>[5x]GPAMGYARRVMDGIGEVAVTGAGGSVTGARLRHQVRLLAHALTEAGIPPGRGVACLHANTWRAIALRLAVQAIGCHYVGLRPTAAVTEQARAIAAADSAALVFEPSVEARAADLLERVSVPVVLSLGPTSRGRDILAASVPEGTPLRYREHPEGIAVVAFTSGTTGTPK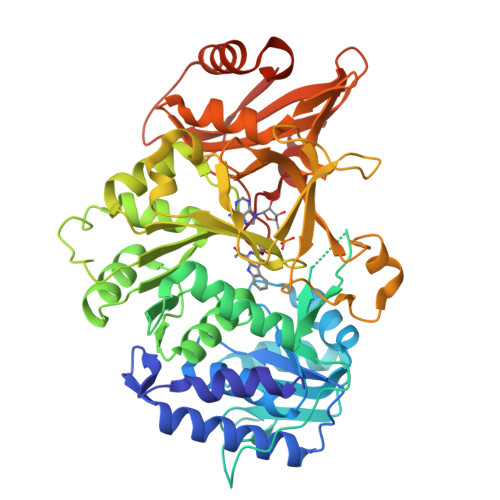GVAHSSTAMSACVDAAVSMYGRGPWRFLIPIPLSDLGGELAQCTLATGGTVVLLEEFQPDAVLEAIERERATHVFLAPNWLYQLAEHPALPRSDLSSLRRVVYGGAPAVPSRVAAARERMGAVLMQNYGTQEAAFIAALTPDDHARRELLTAVGRPLPHVEVEIRDDSGGTLPRGAVGEVWVRSPMTMSGYWRDPERTAQVLSGGWLRTGDVGTFDEDGHLHLTDRLQDIIIVEAYNVYSRRVEHVLTEHPDVRAAAVVGVPDPDSGEAVCAAVVVADGADPDPEHLRALVRDHLGDLHVPRRVEFVRSIPVTPAGKPDKVKVRTWFTD> GPGSGSEGKRL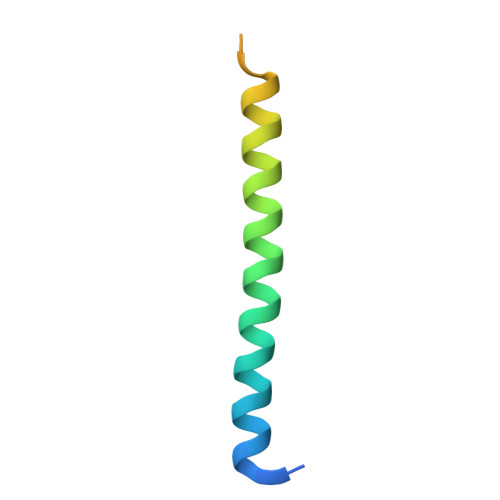TDQLRWKIMSLKMRIEQLKQTISKLNEEMKKNSEGLLKNKEKNQKLYSR>HHHHHHSSGLVPRGSHMQTTTVYSLEDLLPYLKQDNVDVKLAPGTYNVNGFDVGEDRLFSTTPLFLFEGSNSTYDFTDVKLNINTVVLTKFGNNEVNEIQILGNNNVLKNLKLEDIGTTAPSNRAQSIVIDGRDNRIEGFHLTIRGSYPYGYGDAFGKGGGSVINHRKHSGVLIRGLRNHLKDCTIISRSYGHIVAMQAASYPTVEGCYIEGEMRSTDDMLAEEGTGSPADKVDFMTVWGYKLPAGYMMSLQEGGIRAYNAGTTYIDGVEIQRATDNPTVLNCTIK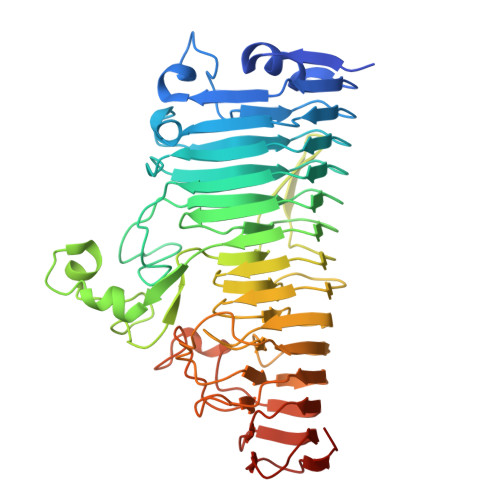NARTGVTLAHANGTKYVEGCTVLGCENGYSIGSGTVVNCGADAIYGPVFKNTYGSDKGYNADITILPPSDAYYNGHDAVAYIGGSNHNLTFRSEITEIPSNLKIMVSGDLQGLRVLHGSNPSQNNFAGTNIVLRNLTNFPVDLHSDSSNITVTSCDTDNITDNGTNNSIEAIDCDSD[2x]> M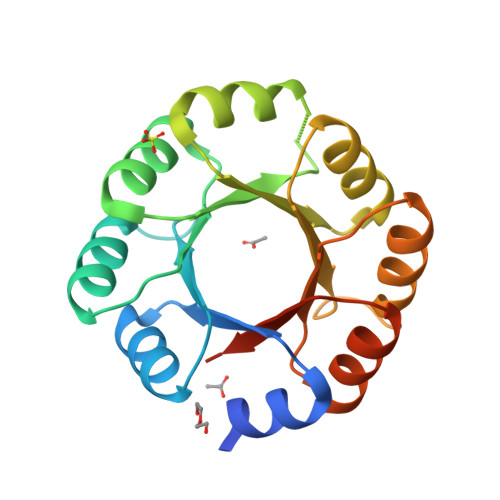DKDEAWKQVEILRRLGAKRIAYRSDDWRDLQEALKKGADILIVDATDKDEAWKQVEILRRLGAKEIAYRSDDWRDLQEALKKGADILIVDATDKDEAWKQVEILRRLGAKRIAYRSDDWRDLQEALKKGADILIVDATDKDEAWKQVEILRRLGAKEIAYRSDDWRDLQEALKKGADILIVDATGLEHHHHHH>[2x]GSHMDGTEKWRFKTGKAIEASPVIGEDGTIYVGSNDGHLYAINPDGTEKWRFKTGKAIEASPVIGEDGTIYVGSND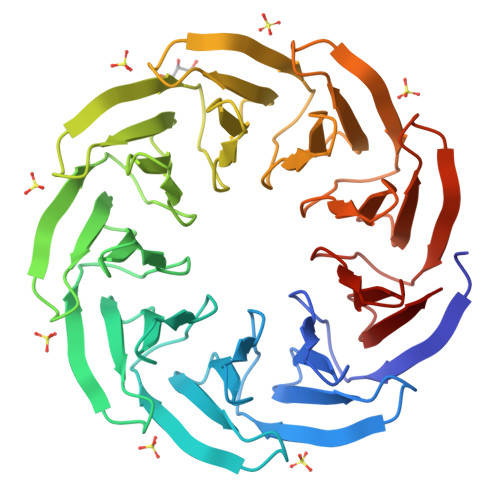GHLYAINPDGTEKWRFKTGKAIEASPVIGEDGTIYVGSNDGHLYAINPDGTEKWRFKTGKAIEASPVIGEDGTIYVGSNDGHLYAINPDGTEKWRFKTGKAIEASPVIGEDGTIYVGSNDGHLYAINPDGTEKWRFKTGKAIEASPVIGEDGTIYVGSNDGHLYAINPDGTEKWRFKTGKAIEASPVIGEDGTIYVGSNDGHLYAINPDGTEKWRFKTGKAIEASPVIGEDGTIYVGSNDGHLYAINPDGTEKWRFKTGKAIEASPVIGEDGTIYVGSNDGHLYAINP> LTPDQQTLLHFIMDSYNKQRMPQEITNKILKEEFSAEENFLILTEMATNHVQVLVEFTKKLPGFQTLDHEDQIALLKGSAVEAMFLRSAEIFNKKLPSGHSDLLEERIRNSGISDEYITPMFSFYKSIGELKMTQEEYALLTAIVILSPDRQYIKDREAVEKLQ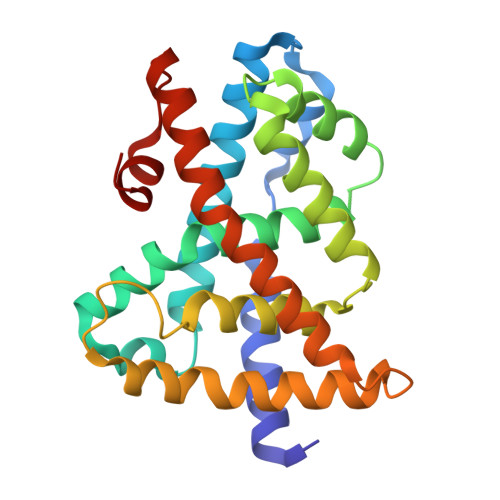EPLLDVLQKLCKIHQPENPQHFACLLGRLTELRTFNHHHAEMLMSWRVNDHKFTPLLCEIWDV9-O-acetyl-5-acetamido-3,5-dideoxy-D-glycero-alpha-D-galacto-non-2-ulopyranosonic 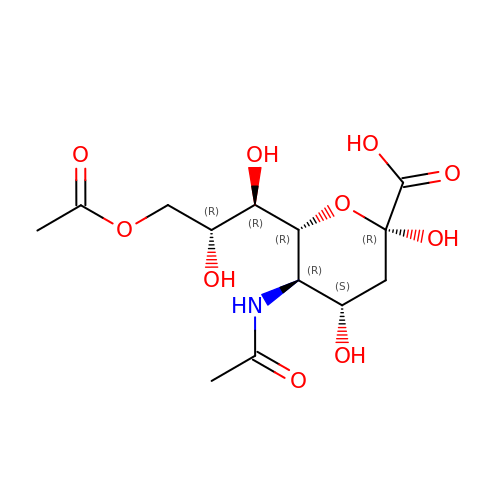acid | C13 H21 N O10 | NYWZBRWKDRMPAS-CTAKWSDESA-N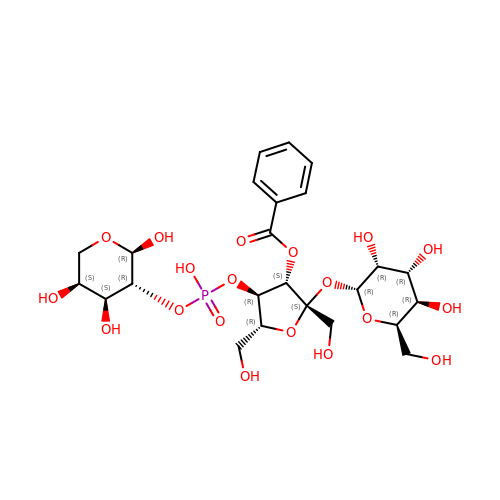[(2S,3S,4R,5R)-2,5-bis(hydroxymethyl)-2-[(2R,3R,4R,5R,6R)-6-(hydroxymethyl)-3,4,5-tris(oxidanyl)oxan-2-yl]oxy-4-[oxidanyl-[(2R,3R,4S,5S)-2,4,5-tris(oxidanyl)oxan-3-yl]oxy-phosphoryl]oxy-oxolan-3-yl] benzoate | C24 H35 O19 P | LMASXRQPXQBKBC-GJRQBPJOSA-N>[3x]XAPAAAAQAV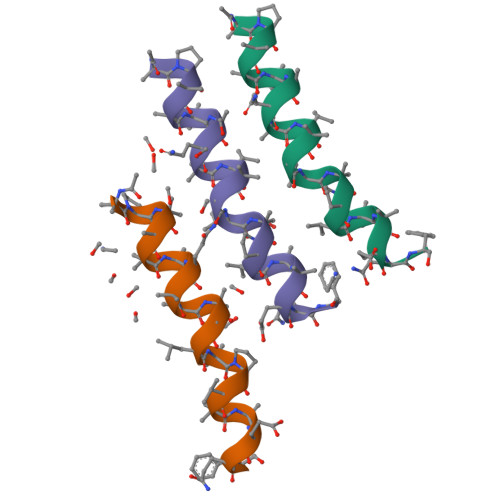AGLAPVAAEQF> GSDNIISFDHVTFTYPDSPRPALSDLSFAIERGSWTALIGHNGSGKSTVSKLINGLLAPDDLDKSSITVDGVKLGADTVWEVREKVGIVFQNPDNQFVGATVSDDVAFGLENRAVPRPEMLKIVAQAVADVGMADYADSEPSNLSGGQKQRVAIAGILAVKPQVIILDESTSMLDPEGKEQILDLVRKIKEDNNLTVISITHDLEEAAGADQVLVLDDGQLLDQGKPEEIFPKVEMLKRIGLDIPFVYRLKQLLKERGIVLPDEIDDDEKLVQSLWQLNSKM;> MAIKFENVSYVYSPGSPLEAIGLDQLNFSLEEGKFIALVGHTGSGKSTLMQHFNALLKPTSGKIEIAGYTITPETGNKGLKDLRRKVSLAFQFSEAQLFENTVLKDVEYGPRNFGFSEDEAREAALKWLKKVGLKDDLIEHSPFDLSGGQMRRVALAGVLAYEPEIICLDEPAAGLDPMGRLEMMQLFKDYQAAGHTVILVTHNMDDVADYADDVLALEHGRLIKHASPKEVFKDSEWLQKHHLAEPRSARFAAKLEAAGLKLPGQPLTMPELADAIKQSLKGGEHE;> MSKIIIGRYLPGTTFVYRVDPRAKLLTTFYFIIMIFLANNWVSYLVISIFGLAYVFATGLKARVFWDGVKPMIWMIVFTSLLQTFFMAGGKVYWHWWIFTLSSEGLINGLYVFIRFAMIILVSTVMTVTTKPLEIADAMEWMLTPLKLFKVNVGM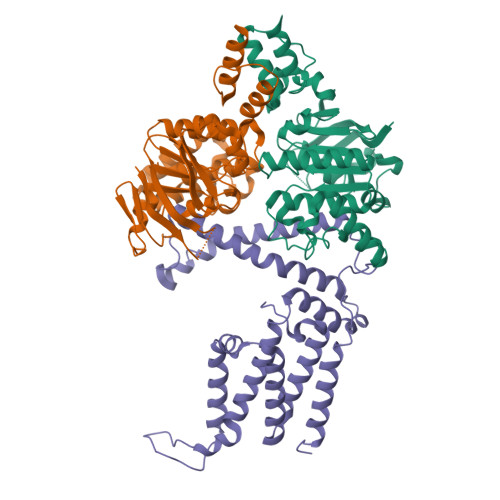ISLVISIALRFVPTLFDQTVKIMNAQRSRGADFNDGGLVKRAKSVVPMLVPLFIDSLEVALDLSTAMESRGYKGSEGRTRYRILEWSKVDLIPVAYCLLLTILMITTRKH> GPHMTVLSDSAHFDVKHPLNTAWTLWYTK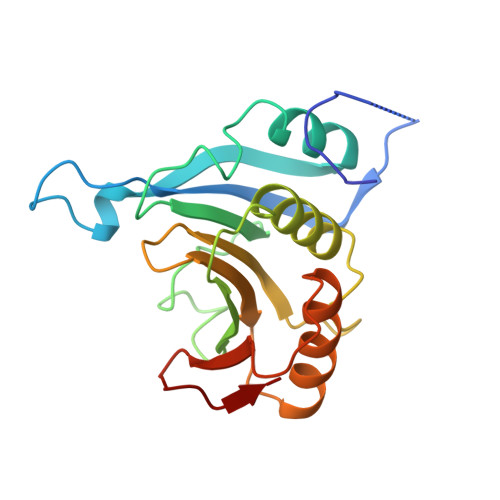PAVDKSESWSDLLRPVTSFQTVEEFWAIIQNIPEPHELPLKSDYHVFRNDVRPEWEDEANAKGGKWSFQLRGAGADIDELWLRTLLAVIGETIDEDDSQINGVVLSIRKGGNKFALWTASEDKEPLLRIGGKFKQVLALTDDGHLEFFPHSSANGRHPQPSITL> GSSVVVDTNGQPVSNGADAYYLVPVSHGHAGLALAKIGNEAE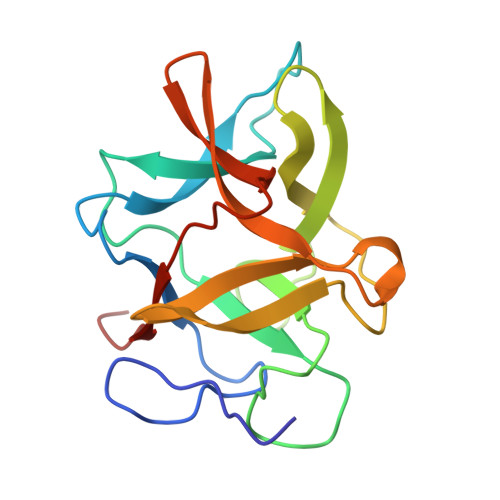PRAVVLDPHHRPGLPVRFESPLRINIIKESYFLNIKFGPSSSDSGVWDVIQQDPIGLAVKVTDTKSLLGPFKVEKEGEGYKIVYYPERGQTGLDIGLVHRNDKYYLAVKDGEPCVFKIRKATDE>ETGSAQQLNEDLRLHLLLNTSVTCNDGSPAGYYLKESRGSRRWLLFLEGGWYCFNRENCDSRYDTMRRLMSSRDWPRTRTGTGILSSQPEENPYWWNANMVFIPYCSSDVWSGASSKSEKNEYAFMGALIIQEVVRELLGRGLSGAKVLLLAGSAAGGTGVLLNVDRVAEQLEKLGYPAIQVRGLADSGWFLDNKQYRHTDCVDTITCAPTEAIRRGIRYWNGVVPERCRRQFQEGEEWNCFFGYKVYPTLRSPVFVVQWLFDEAQLTVDNVHLTGQPVQEGLRLYIQNLGRELRH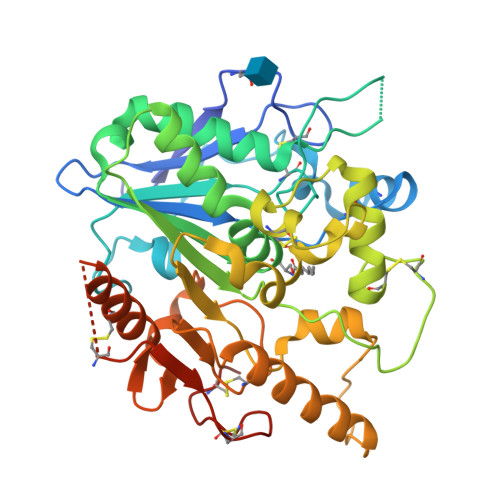TLKDVPASFAPACLSHEIIIRSHWTDVQVKGTSLPRALHCWDRSLHDSHKASKTPLKGCPVHLVDSCPWPHCNPSCPTGTKHHHHHH[2x]> ASAAEELQKSIGHKPEPTDEEWELIKTVTEAHVATNAQGSHWKQKR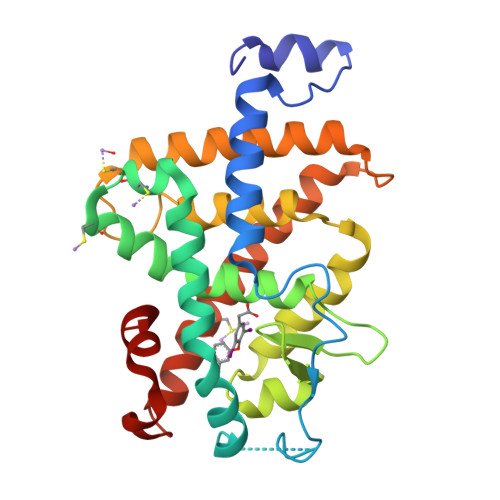KFLPEDIGQAPIVNAPEGGKVDLEAFSHFTKIITPAITRVVDFAKKLPMFCELPCEDQIILLKGCCMEIMSLRTAVRYEPESETLTLNGEMAVTRGQLKNGGLGVVSDAIFDLGMSLSSFNLDDTEVALLQAVLLMSSDRPGLACVERIEKYQDSFLLAFEHYINYRKHHVTHFWPKLLMKVTDLRMIGACHASRFLHMKVECPTELFPPLFLEVFED{2-[1-(6,7-dimethoxyquinazolin-4-yl)piperidin-4-yl]ethyl}phosphonic 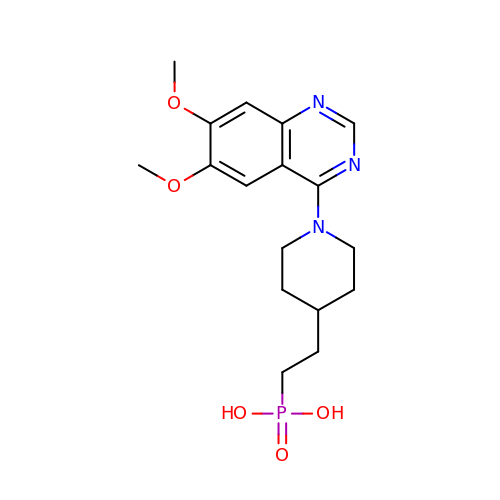acid | C17 H24 N3 O5 P | SNLWMWQNJTVWKD-UHFFFAOYSA-N> MVEATAQETDRPRFSFSIAAREGKARTGTIEMKRGVIRTPAFMPVGTAATVKALKPETVRATGADIILGNTYHLMLRPGAERIAKLGGLHSFMGWDRPILTDSGGYQVMSLSSLTKQSEEGVTFKSHLDGSRHMLSPERSIEIQHLLGSDIVMAFDECTPYPATPSRAASSMERSMRWAKRSRDAFDSRKEQAENAALFGIQQGSVFENLRQQSADALAEIGFDGYAVGGLAVGEGQDEMFRVLDFSVPMLPDDKPHYLMGVGKPDDIVGAVERGIDMFDCVLPTRSGRNGQAFTWDGPINIR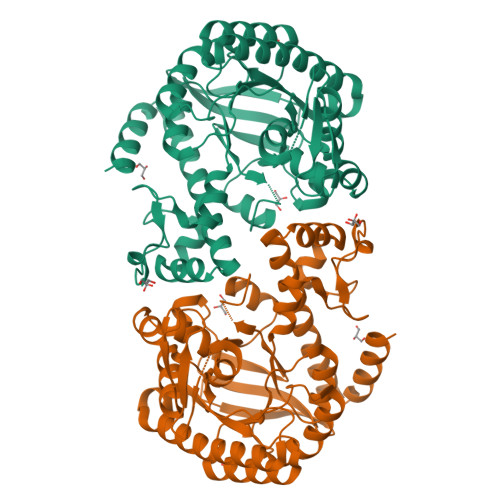NARFSEDLKPLDSECHCAVCQKWSRAYIHALIRAGEILGAMLMTEHNIAFYQQLMQKIRDSISEGRFSQFAQDFRARYFARNS>MGSSHHHHHHSSGLVPRGSHSYFDDSVAIVGISCQFPGAKNHHEFWKQLREGKESVRFYSEEELREAGVPEDLIENPDYVPALSTIEG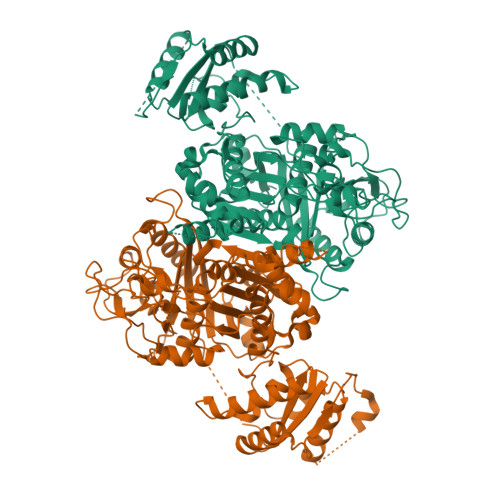KDLFDPEFFHISPKDAEFMDPQLRLLLLHSWKAVEDAGYVSKEIPKTSVYMSASNNSYRSLLPEKTTEGHESPDGYVSWVLAQSGTIPTMVSHKLGLKGPSYFVHSNCSSSLVGLYSAYKSITSGESEYALVGGATLHAATSIGYVHQNGLNFSSDGHVKAFDASADGMAGGEGAAVILLKKASQAVQDGDHIYAMLRGIGLNNDGADKVGFYAPSVKGQTDVIQHVLDSTNIHPETISYIEAHGTGTTLGDPIEMSALQQVYKRYTDREQYCGIGSVKTNIGHLDTAAGLAGCIKVAMSLYHRELAPTINYTSPNPNIKFSGSPFYVADKRKTLPERETPHRAALSSFGLGGTNAHAIFEQYENKTISGSNDGQPPYIVPLSARNKQRLTAYASCLSGFLDEAENDVSLHDLAYTYQTGREAMEERAVFISHDRHDLNRQLQDFINGNDQNILRGEKVRSREVSAQEMEELAACQTRDEKLKALAALWVEGARVDWGLLYPDSAPQRISAPTYPFAEERFWPEETVK[2x]> SGRFDQYPTKKGDFAIDG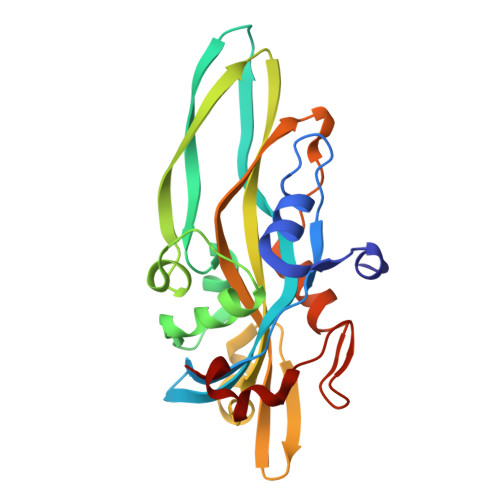YLLDYSSPKQGCWVDGITVYGDIYIGKQNWGTYTRPVFAYLQYVETISIPQNVTTTLSYQLTKGHTRSFETSVNAKYSVGANIDIVNVGSEISTGFTRSESWSTTQSFTDTTEMKGPGTFVIYQVVLVYAHNATSAGRQNANAFAYSKTQAVGSRVDLYYLSAITQRKRVIVPSSNAVTPLDWDTVQRNVLMENYNPGSNSGHFSFDWSAYNDPHRRY>MCPTLNNIVSSLQRNGIFINSLIAALTIGGQQLFSSSTFSCPCQVGKNFYYGSAFLVIPALILLVAGFALRSQMWTITGEYCCSCAPPYRRISPLECKLACLRFFSITGRAVIAPLTWLAVTLLTGTYYECAASEFASVDHYPMFDNVSASKREEILAGFPCCRSAPSDVILVRDEIALLHRYQSQMLGWILITLATIAALVSCCVAKCCSPLTSLQHCYWTSHLQNERELFEQAAEQHSRLLMMHRIKKLFGFIPGSEDVKHIRIPSCQDWKDISVPTLLCMGDDLQGHYSFLGNRVDEDNEEDRSRGIELKP[22x]

In humans, the CALHM family encompasses six paralogs, some of which function as non-selective channels that are permeable to large substances such as ATP. We identified the three paralogs, CALHM2, 4 and 6, to be highly expressed in this organ. The CALHM subunits thus constitute unique modular building blocks that assemble with different stoichiometries into large membrane channels. In contrast to previously described CALHM structures, where the oligomeric state of individual channels was described as uniform, our data show heterogeneous populations with CALHM4 and CALHM6 assembling as decameric and undecameric channels with similar abundance and CALHM2 as predominantly undecameric proteins with a smaller population of dodecamers (Figure 3—figure supplements 2–4 and 6). Despite the unknown activating stimuli, our study has provided insight into gating transitions of CALHM channels by showing two conformations with either a cylindrical pore of uniform large dimeter within the membrane that is constricted at the intracellular side as in case of CALHM4 and a conical pore that continuously narrows from its extracellular entry towards the cytoplasm as in case of CALHM6.

The smaller particles are composed of decameric and the larger of undecameric assemblies, both of which we refer to as CALHM4 channels. Due to the slightly higher quality of the Ca2+-free sample, we continued to use this data for our further analysis unless specifically indicated. The cryo-EM density of the decamers extends to a resolution of 4.1 Å and undecamers to 3.7 Å, which in both cases permitted the unambiguous interpretation by an atomic model (Figure 3—figure supplements 2, 3 and 5A). In each structure, the subunits are arranged around a central axis of symmetry that defines the ion-conduction path. Both assemblies contain pairs of CALHM4 channels of the same size related by two-fold symmetry that interact via their cytoplasmic parts. In the plane of the membrane, the dimensions of decameric and undecameric CALHM4 channels amount to 110 Å and 120 Å respectively. The diameter at both entrances of the pore measures about 52 Å and 60 Å for decameric and undecameric assemblies respectively, thus defining the properties of an unusually large channel, which could be permeable to molecular substrates. Even at the constriction located at the intracellular membrane leaflet where the respective N-terminal helices NH project towards the pore axis, the decameric channels are about 20 Å and undecameric channels 30 Å wide. In our data, we find strong evidence for a layered distribution of density inside the pore within the presumed membrane region in non-symmetrized maps and after application of symmetry. This density is observed with similar properties in decameric and undecameric proteins in both datasets of CALHM4 obtained in either absence or presence of Ca2+.Specific insect behaviors can be stimulated after recognizing chemicals in the external environment through conserved chemosensory proteins (CSPs) in chemoreceptive organs, which are critical components of the olfactory systems. CSPs are present in chemoreceptive organs and can bind a range of aliphatic compounds, esters, and other long-chain compounds to stimulate specific insect behaviors. CSPs consist of 100–115 amino acids with molecular weights of ~13 kDa. To explore its structural basis for ligand-recognizing capability, we solved the 2.3 Å crystal structure of the apoprotein of S. litura CSP8 (SlCSP8).

Therefore, we only worked on the truncated version D18-E128 for the follow-up structural and biochemical studies. The protein was crystallized in the space group of P212121 and each asymmetric unit contains a single molecule. The cloned fragment is completely visible, in addition to the C-terminal 6× His tag (the last histidine residue is missing). The N-terminal residues V17-D26 form a flexible loop, followed by six helices (N27–N122), which form the main body of the structure. The C-terminal tag adds an additional helix (α7) and extends to the solvent. The helices of the main body collapse onto each other and form a small central channel. α6 is parallel to the two planes formed by α2–α3 and α4-α5, respectively, but is perpendicular to α4. Two disulfide bonds are formed between C72 and C75, between C46 and C53, respectively. The overall structure is spherical, with the surface charges of the protein being mainly negative. The closest structural homolog apo-MbCSPA6 (78% sequence identity) could be aligned onto SlCSP8 with an RMSD of 0.96 Å over 100 Cα atoms, suggesting a high structural resemblance. Our results showed that the SlCSP8 protein has the highest and lowest affinities to rhodojaponin III and avermectin, respectively, while it displays moderate affinities to 12-bromododecanol and bombykol, with the former being a better binder than the latter.

> VDEKYPSKYDNIDLDEILANKRLLTAYVNCIMERGKCSPEGKELKEHLVDAIETGCSKCTEAQEKGAYKVIEHLIQNELDTWHELTDKYDSSGKWRKTYEDRARANGIVIPELEHHHHHH> GAMGNQTVKIWVKYNEGF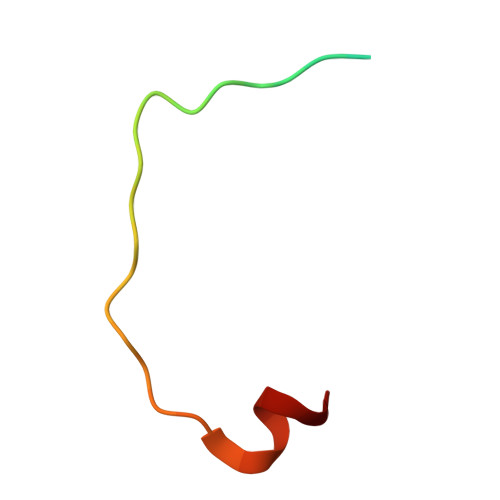SNAVRKNVTWNNLWE>[2x]MAETAIVTKSENPHIVILPSPGMGHLIPLVEFSKRLISQHQFSVTLILPTDGPISNSQKSFLNSLPSCMDYHLLPPVNFDDLPLDVKIETRISLTVTR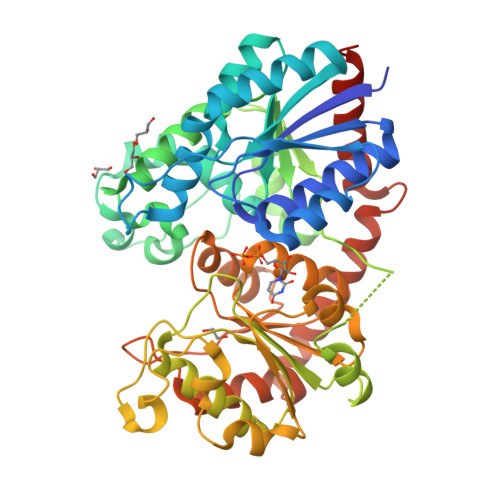SLSSLREVFKTLVDSKKVVAFVVDLFGTDAFDVAIDFNVSPYIFFPSTAMALSLFLYLPKLDATVSCEYRDLPDPIQIPGCIPIHGKDLLDPVQDRKNEAYRWLLHHSKRYRMAEGVVSNSFKELEGGPIKALQEEEPGKPPVYPVGPLIQMDSGSKVDGSGCLTWLDEQPRGSVLYVSYGSGGTLSHEQLIEVASGLEMSEQRFLWVIRCPNDTVANATYFNVQDSTNPLDFLPKGFLERTKGLGLVVPNWAPQAQILSHGSTGGFLTHCGWNSTLESVVHGVPLIAWPLYAEQKMNAVMLTEDIKVALRPKANENGLVGRLEIAKVVKGLMEGEEGKGVRTRMRDLKDAAAKVLSQDGSSTKALAELATKLKNKVLINGSENLYFQ>EQIGGSVITDVDLTRRLLPGDGPGEFFLPPLPRLLPAGYHPDAARIEIASNGWVRRMLADCFDSEESLLFFLRQRNGIYGPLTVPYAEADRAQNIADWYQFVTVIDSFVSDEAALGADHAAAAETFAAVVADLREGGAGGPAASLYGRAAQDLWRRIAAGMSARQVDRLVAALEAFLRGCAEEIRSKLDKQVPHFEACMRVRVDSFGCEFLELLTEYAAEVDMSRAATEGLFDEVHHHGMRQLILVNDLLSWRKEYAQRDTMTTVRVLCEVEGLELQDAVDRLCALVEHHERAYITARDAVLAGPHGHREDVRAYLSGLDHLIGGSQEFEYLTPRYFGDGSVWDGSTSGWISLTASVARFRDAPAPAPSARPTRPLV[2x]

Diterpene synthase VenA is responsible for assembling venezuelaene A with a unique 5-5-6-7 tetracyclic skeleton from geranylgeranyl pyrophosphate. VenA also demonstrates substrate promiscuity by accepting geranyl pyrophosphate and farnesyl pyrophosphate as alternative substrates. A promiscuous DTS VenA containing an atypical 115DSFVSD120 motif was characterized to catalyze the unique cyclization of geranylgeranyl pyrophosphate (GGPP, C20), giving rise to 1. The monomer of VenA holds a typical isoprenoid synthase α-fold comprised of twelve core α-helices and four additional short α-helices.

In the PPi-(Mg2+)3-bound form, a trinuclear magnesium cluster is coordinated in an octahedral manner by the conserved amino acid residues in the Asp-rich and NSE motifs, PPi group and water molecules. Specifically, Mg2+A and Mg2+C are coordinated by ten oxygen atoms of Asp115, PPi group, and surrounding water molecules on the same side of the active site. In the opposite side of the active site, Mg2+B is coordinated by six oxygen atoms of NSE triad (Asn256, Ser260 and Glu264), PPi group, and one water molecule. The hydrogen bonds between coordinated water molecules and Glu192, Ser214, and Asp257 were also observed in the PPi-(Mg2+)3-bound form of VenA. Upon coordination with the trinuclear magnesium cluster, Asp115 and NSE motif stretch towards the active site and lead to the movement of C and H helices, which reduces the volume of substrate binding cavity. Meanwhile, the PPi group forms a number of hydrogen bonds with the “PPi sensor” residues Arg211 and Lys263 in the NSE motif, and the 344RY345 dimer in the active site of VenA, which play crucial roles in substrate trapping and conversion. Besides the amino acid residues in metal-binding motifs, Arg344 and Tyr108 in the active site of PPi-(Mg2+)3-bound VenA rotate by a wide margin compared with those in apo form. Meanwhile, the guanidine group of Arg344 is rotated towards the PPi group, thereby forming a hydrogen bond. Ser116 and Gln83 in the PPi-(Mg2+)3-bound form may help maintaining the hydrophobic catalytic pocket by interacting with Arg344. The results clearly indicated that only the first Asp115 is required for VenA’s activity; supporting this, Asp120 was found to be located outside of the active site and far from the PPi group (9.4 Å), Mg2+A (7.9 Å) and Mg2+C (9.1 Å).> MTAPPDLRVVCHRLASTPVDSLPRLCPLLINHVLRCGGPLSEPQDAKGKDRTSETAMLVHKFRTHITSLLTGKSPAGRFTAVCLIKAVIDVGGWESLRSAEPWIRGLIGVLQKPDPLSSKELSIVTLTKLYILLQDYQTLIREMATPTLPGYATACLQLIKPPASGRPLKVPLNFVDTVAWSLSKLVVLYSTTMRPFSGQIKSALRPYIAPTSSDNVVVPQSLKENSRNLLILLTYTAPKNGSSDEWVKAIRATILDCHTTADQVFRAVRESWESTTGYHIQPVNATGEPSGGGDSVDELPPWSGLQAGAERLTGLLEYLTAYFNNPTRAPVNVPLGELLDLTTRLTLVIPPSLGAEDSIETNPAIGRDEKAELWSALPDIHHAVLRLHCAIIRRLEANAIPLATDIIDQMVRVSTASKQLPSVRETAYILAKEIL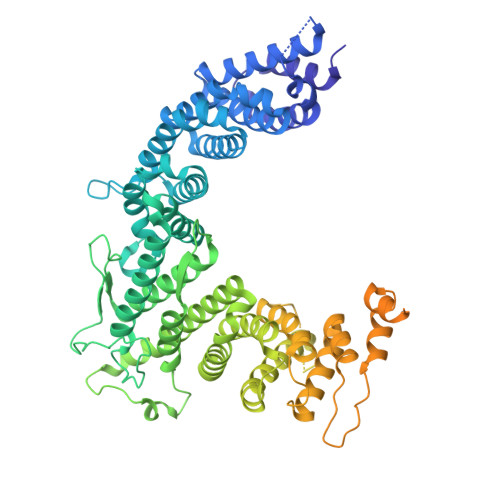LLAGSTLPKLTVDILIPLIQSSCHDILTAAGHAQPAQSQSSVPVTASKQQKSSSPALTNADAFLPGQSSSSTPKTSTASPVSQAASALLPTFFTHLPQKHLPPDIRGLLDRTAILSHNQSAMLASCLHPYRDSRGRYYPSILPFLVRRFPRDESVEVLRSNLVKVGGSDASRGWDLSNGVTRDISYGREFAQEMISEEKGVVKEDETFAKEIEPVKSTAKPATSANAWGVEMELDVEHVNVAPIPETTNPFATVVGTTSQPSTLIQPACPSSPLKRKSDAEEFDEGSRPKRVDTGKAVSHPQMAVISSVPKPEEDKSDESSDSEGSVQIDMTLEDDEEDEEEEDE> MAFSADTSEIVYTHDTGLDYITYSDYELDPANPLAGGAAWIEGAFVPPSEARISIFDQGYLHSDVTYTVFHVWNGNAFRLDDHIERLFSNAESMRIIPPLTQDEVKEIALELVAKTELREAFVSVSITRGYSSTPGERDITKHRPQVYMYAVPYQWIVPFDRIRDGVHAMVAQSVRRTPRSSIDPQVKNFQWGDLIRAVQETHDRGFEAPLLLDGDGLLAEGSGFNVVVIKDGVVRSP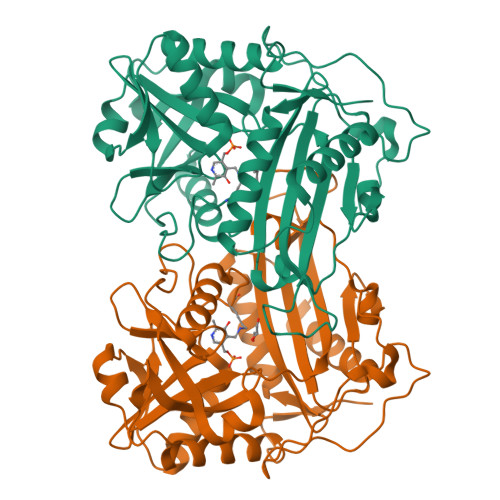GRAALPGITRKTVLEIAESLGHEAILADITLAELLDADEVLGCTTAGGVWPFVSVDGNPISDGVPGPITQSIIRRYWELNVESSSLLTPVQY>[2x]MQRREFLKLSALGVGAMALRGSGPAKALKAPWYAQEVKSVYQICEGCFWRCGIVAHAVGNRVYKVEGYEANPKSRGRLCPRGQGAPQTTYDPDRLKRPLIRVEGSQRGEGKYRVATWEEALDHIAKKMLEIREKYGPEAIAFFGHGTGDYWFVDFLPAAWGSPNAAKPSVSLCTAPREVASQWVFGRPIGGHEPIDWENARYIVLIGHHIGEDTHNTQLQDFALALKNGAKVVVVDPRFSTAAAKAHRWLPIKPGTDTALLLAWIHVLIYEDLYDKEYVAKYTVGFEELKAHVKDFTPEWAEKHTEIPAQVIREVAREMAAHKPRAVLPPTRHNVWYGDDTYRVMALLYVNVLLGNYGRPGGFYIAQSPYLEKYPLPPLPLEPAAGGCSGPSGGDHEPEGFKPRADKGKFFARSTAIQELIEPMITGEPYPIKGLFAYGINLFHSIPNVPRTKEALKNLDLYVAIDVLPQEHVMWADVILPEATYLERYDDFVLVAHKTPFIQLRTPAHEPLFDTKPGWWIARELGLRLGLEQYFPWKTIEEYLETRLQSLGLDLETMKGMGTLVQRGKPWLEDWEKEGRLPFGTASGKIELYCQRFKEAGHQPLPVFTPPEEPPEGFYRLLYGRSPVHTFARTQNNWVLMEMDPENEVWIHKEEAKRLGLKEGDYVMLVNQDGVKEGPVRVKPTARIRKDCVYIVHGFGHKAPLMRLAHGRGASDNYLQTRYKLDPISGGAGLRVNFVRLEKAERPRLPSLTGLAKRPFDERRM;>MPRYAMAIDLSLCVGCAACAVACKMENEVPPGVFNLW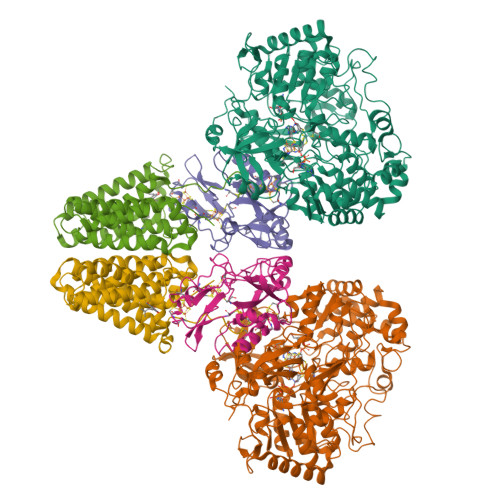IREREVGEYPNLVVEFRPEQCLHCENPPCVPVCPTGASYQTKDGLVLVDPKKCIACGACIAACPYDARYLHPAGYVSKCTFCAHRLEKGKVPACVETCPTYCRTFGDLEDPESPVAKALKAAERVDVLRPEQGTRPKLFYLNAPSKKGLTRESEVHHG[2x];>MAEFYGLPNAQEFWHWTNALHFVLVGLAGGVALLAALLHLKGDAEARRYTLYALMLIALDLFILWAESPARFRFTHIWLFLSFHPTSPIWWGAWGLGLGFLTGGLLYLGKGSQRALAWALLVFSLVALSYPGLALAVNLNRPLWNGLMAGLFPLTALVLALGLAALLKSPWALFPLRVLAGASLLLALLYPLTLPPEARGHLLEEAGFWYGLFLLLGLGTFWQERLAPWAGLLAAAGLRALLVLAGQWQGLGL[2x]> GPQSEPELKLESVVIVSRHGVRAPTKATQLMQDVTPDAWPTWPVKLGWLTPRGGELIAYLGHYQRQRLVADGLLAKKGCPQSGQVAIIADVDERTRKTGEAFAAGLAPDCAITVHTQADTSSPDPLFNPLKTGVCQLDNANVTDAILSRAGGSIADFTGHRQTAFRELERVLNFPQSNLCLKREKQDESCSLTQALPSELKVSADNVSLTGAVSLASMLTEIFLLQQAQGMPEPGWGRITDSHQWNTLLSLHNAQFYLLQRTPEVARSRATPLLDLIKTALTPHPPQKQAYGVTLPTSVLFIAGHATNLANLGGALELNWTLPGQPDNTPPGGELVFERWRRLSDNSQWIQVSLVFQTLQQMRDKTPLSLNTPPGEVKLTLAGCEERNAQGMCSLAGFTQIVNEARIPACSL

AppA, the Escherichia coli periplasmic phytase of clade 2 of the histidine phosphatase (HP2) family, has been well-characterized and successfully engineered for use as an animal feed supplement. The E. Coli periplasmic phytase, AppA, is a 1D-6-phytase (EC 3.1.3.2) and initial hydrolysis preferentially liberates the phosphate at the 1D-6-position on the inositol ring. HP2Ps catalyse the hydrolysis of phytate via an obligatory phosphohistidine intermediate. The catalytic proton donor is found in a second, short, conserved motif with sequence HD positioned such that the aspartic acid residue functions as the consensus proton donor in the catalytic mechanism.

While the wild-type enzyme has a strong preference for 1D-6-phytase activity, a marked reduction in stereospecificity was observed for a D304E variant, while a proton donor-less mutant (D304A) displayed exclusive 1D-1/3-phytase activity. Notably, KM was 5-fold lower than wild type for the proton donor-less AppA-HAT variant and the MINPP-like AppA-HAE double mutant. On the other hand, action of the AppA-HAT variant revealed a reversal of stereospecificity from the wild-type enzyme generating InsP5 [1/3-OH] equivalent to 89% of the total InsP5s. Turning first to variants bearing mutations at position 304, substitution of the proton donor residue with an alanine (AppA-HAT) leads to an increase in volume of specificity pockets A and B and a shift of the inhibitor (rmsd 0.5 Å for carbons of the inositol ring) towards pocket B. A modest shift is also observed in the conformations of the sidechains of pocket B residues, His250 and Phe254. This variant shows a marked change in stereospecificity displaying almost exclusive ID-1/3-phytase activity. Indeed, this provides evidence for an intrinsic role played by the proton donor residue itself in determining the stereospecificity of the enzyme. Although we did not determine the absolute enantiomerism of the InsP5 product, placing the 1D-1- or 1D-3-phosphate in pocket A results in the axial 2-phosphate occupying pockets B or F, respectively. In the absence of further evidence, the increased size of pocket B following the D304A mutation may point to an enhanced 1-phytase activity of this proton donor-less variant. Why for this variant the inhibitor binds with the 1D-6-sulfate in specificity pocket A rather than the 1D-1- or 1D-3-sulfate as suggested by the results of HPLC analysis is unclear; however, we note that a previous crystallographic study of a variant AppA resulted in a similar phenomenon.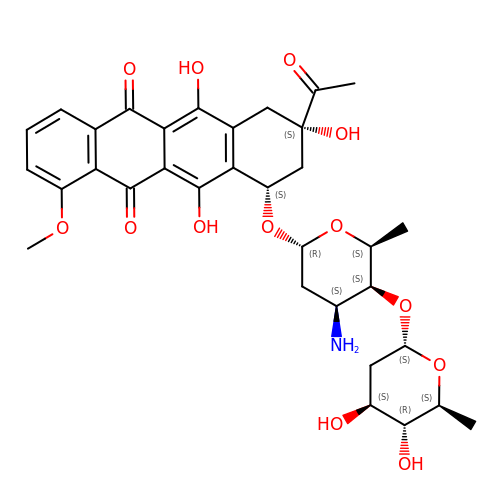4'-EPI-4'-(2-DEOXYFUCOSE)DAUNOMYCIN | C33 H39 N O13 | QTGKDZKONUUXOU-NIGIIATCSA-N>AVRGSIIANMLQEHDNPFTLYPYDTNYLIYTNTSDLNKEAISTYNWSENARKDEVKFQLSLAFPLWRGILGPNSVLGASYTQKSWWQLSNSKESSPFRETNYEPQLFLGFATDYRFAGWTLRDVEMGYNHDSNGRSDPTSRSWNRLYTRLMAENGNWLVEVKPWYVIGSTDDNPDITKYMGYYQLKIGYHLGEAVLSAKG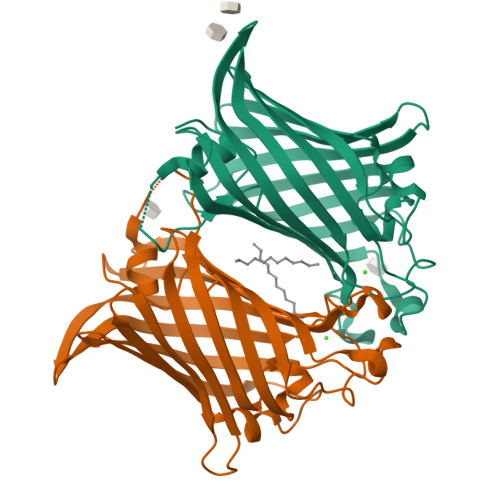QYNWNTGYGGAEVGLSYPVTKHVRLYTQVYSGYGESLIDYNFNQTRVGVGVMLNDIF[2x]> GHHHHHHHENLYFQGLEDLVEDSHA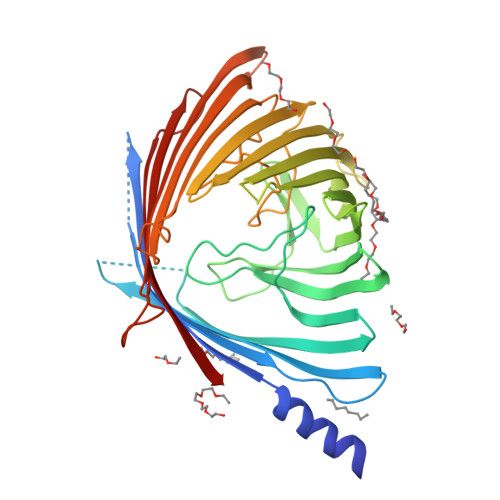SLELRNFYFNRDFRQSGARDNADEWAQGFLLRLESGFSEGTVGFGVDAIGLLGFKLDSGSGSGGTGLLPADGSAGGSQDDYAKLGLTAKARVSNSLLKVGALHFKSPLVSANDTRLLPELFRGALLDVQEIDGLTLRGAHLDRNKLNSSSDYQVFSANRIGGRSDAFDFAGGDYRLTPALTASLHQGRLKDIYRQTFAGLVHTLDLGGQRSLKSDLRFARASEDGGFRELDNRAFGALFSLRLGAHAVAAGYQRISGDDPYPYIAGSDPYLVNFIQIGDFGNVDERSWQLRYDYDFGALGLPGLSFMSRYVSGDNVARGAANDGKEWERNTDLGYVVQSGPLKNLGVKWRNATVRSNFANDLDENRLILSYSLALW> MNENLWKICFIVMFIIWVFVRKV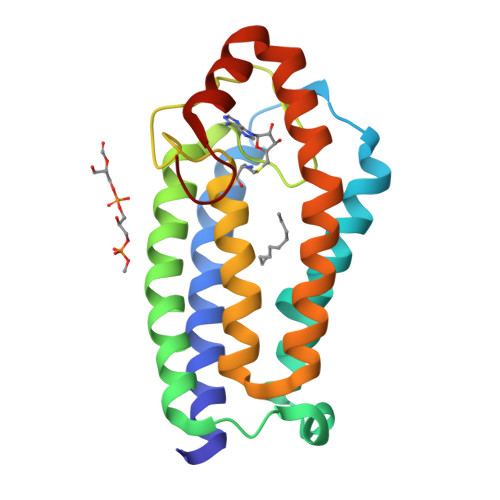YGTRAMKNKSKKKVRPNFEKSLVFLNFIGMVFLPLTAVFSSYLDSFNINLPDSIRLFALIVTFLNIGLFTKIHKDLGNNWSAILEIKDGHKLVKEGIYKNIRHPMYAHLWLWVITQGIILSNWVVLIFGIVAWAILYFIRVPKEEELLIEEFGDEYIEYMGKTGRLFPKVV> MASATTSSKNGKPLVVVYGDYKCPYC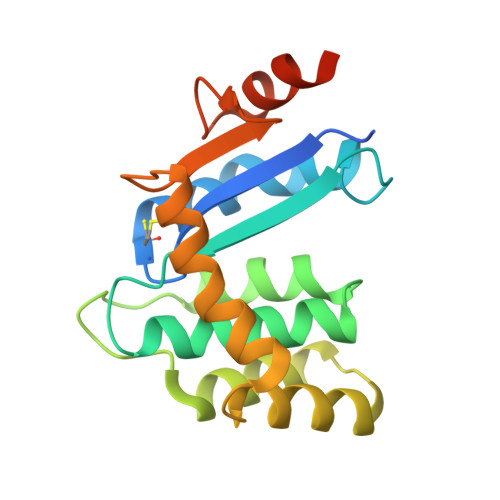KELDEKVMPKLRKNYIDNHKVEYQFVNLAFLGKDSIVGSRASHAVLMYAPKSFLDFQKQLFAAQQDENKEWLTKELLDKHIKQLHLDKETENKIIKDYKTKDSKSWKAAEKDKKIAKDNHIKTVPTAFINGEKVEDPYDYESYEKLLKDKIKLEHHHHHH> MGSSHHHHHHSSGLVPRGSMGTRKKVHAFVRVKPTDDFAHEMIRYGDDKRSIDIHLKKDIRRGVVNNQQTDWSFKLDGVLHDAS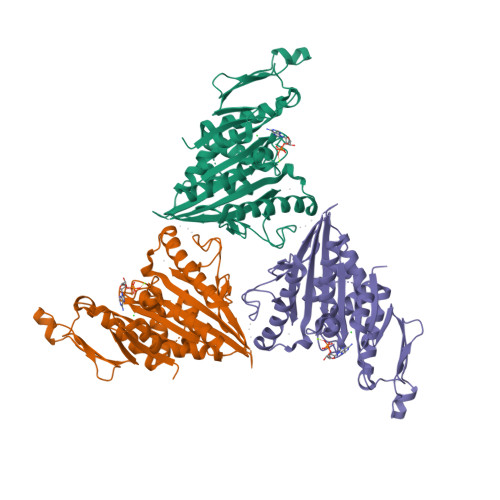QDLVYETVAKDVVSQALDGYNGTIMCYGQTGAGKTYTMMGATENYKHRGILPRALQQVFRMIEERPTHAITVRVSYLEIYNESLFDLLSTLPYVGPSVTPMTIVENPQGVFIKGLSVHLTSQEEDAFSLLFEGETNRIIASHTMNKNSSRSHCIFTIYLEAHSRTLSEEKYITSKINLVDLAGSERLGKSGSEGQVLKEATYINKSLSFLEQAIIALGDQKRDHIPFRQCKLTHALKDSLGGNCNMVLVTNIYGEAAQLEETLSSLRFASRMKLV> FSNNNFVYTDGTHFALNGKSLYINGFNAYWLMYIAYDPSTRIKVTNTFQQASKYKMNVARTWAFSHGGSRPLQSAPGVYNEQMFQGLDFVISEAKKYGIHLIMSLVNNWDAFGGKKQYVEWAVQRGQKLTSDDDFFTNPMVKGFYKNNVKVVLTRVNTITKVAYKDDPTI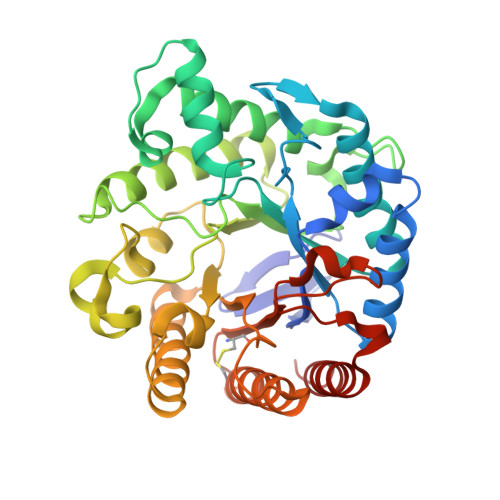LSWELINEPRCPSDLSGKTFQNWVLEMAGYLKSIDSNHLLEIGLEGFYGNDMRQYNPNSYIFGTNFISNNQVQGIDFTTIHMYPNQWLPGLTQEAQDKWASQWIQVHIDDSKMLKKPLLIAEFGKSTKTPGYTVAKRDNYFEKIYGTIFNCAKSGGPCGGGLFWQVLGQGMSSFDDGYQVVLQESPSTSRVILLQSLRLSKLS>[15x]QVIEMNNSPLRDFVTWYSKQTGESVIVSPDVKGTVTVYSSDVKPENLRNFFISVLRANNFDMVGSNPSIIQKYNPNNQDYIDELPSSDNQEYDDNSAPSGGFFVPQNDNVTQTFKINNVRAKDLIRVVELFVKSNTSKSSNVLSVDGSNLLVVSAPKDILDNLPQFLSTVDLPTDQILIEGLIFEVQQGDALDFSFAAGSQRGTVAGGVNTDRLTSVLSSAGGSFGIFNGDVLGLSVRALKTNSHSKILSVPRILTLSGQKGSISVGQNVPFITGRVTGESANVNNPFQTVERQNVGISMSVFPVAMASAHHHHHHHGGNIVLDITIKADSLSSSTQASDVITNQRSIATTVNLRDGQTLLLGGLTDYKNTSQDSGVPFLSKIPLIGLLFSSRSDSNEESTLYVLVKATIVRAL

Instead, new virions are extruded via the phage-encoded pIV protein, which has homology with bacterial secretins. pIV is a secretin family protein, with sequence similarity to bacterial secretins at the core of the Type IV pilus assembly machinery and the Type II and Type III secretion systems. Fifteen f1 pIV subunits assemble to form a gated channel in the bacterial outer membrane, with associated soluble domains projecting into the periplasm. The C-terminal domain integrates into the bacterial outer membrane and forms a double-walled ß-barrel with a central gate forming a stricture at the centre.

We present here the cryoEM structure of the closed state of f1pIV to 2.7 Å resolution, the first near-atomic resolution structure of a phage secretin protein. Averaging the protein particles together in 2D showed that f1pIV particles are composed of fifteen identical subunits; no variation in symmetry was observed. The N-terminal part of f1pIV is comprised of two periplasmic N domains: the far N-terminal N0 domain (residues 1–88) and the N3 domain (108–172), which are joined together with a 19-residue linker (89–107). The fifteen subunits pack against each other to form the secretin channel, with each subunit contributing a four-stranded ß-sheet to the multimer, culminating in a large ß-barrel composed of 60 ß-strands. Within the ß-barrel is a smaller inner barrel comprised of four ß-strands from each f1pIV subunit. The inner ß-barrel is angled parallel to the pore axis and provides a scaffold for two extended loops that reach into the centre of the pore, known as Gate 1 and Gate 220. The interface between the outer and inner ß-barrels is composed mostly of hydrophobic residues, and strengthened further with a salt bridge between Glu 185 and Arg 337 (both residues are highly conserved amongst homologues). The interface between neighbouring N3 domains is mostly hydrophobic, and no hydrogen bond interactions are observed between them in our structure. For reasons of flexibility, the extracellular part of the ß-barrel was missing interpretable density (36 amino acid residues, positions 199–234) as well as the very centre of the pore in the Gate 1 loop (15 residues, positions 275–289). The far N-terminal N0 domain and its associated 19 residue linker region (residues 1–107) could not be observed in our structure. Two molecules of CHAPS were observed to bind to each f1pIV subunit, forming a circle of detergent around the barrel.>[2x]MSKIFDLVVIGAGSGGLEAAWNAATLYKKRVAVIDVQMVHGPPFFSALGGTCVNVGCVPKKLMVTGAQYMEHLRESAGFGWEFDRTTLRAEWKNLIAVKDEAVLNINKSYDEMFRDTEGLEFFLGWGSLESKNVVNVRESADPASAVKERLETEHILLASGSWPHMPNIPGIE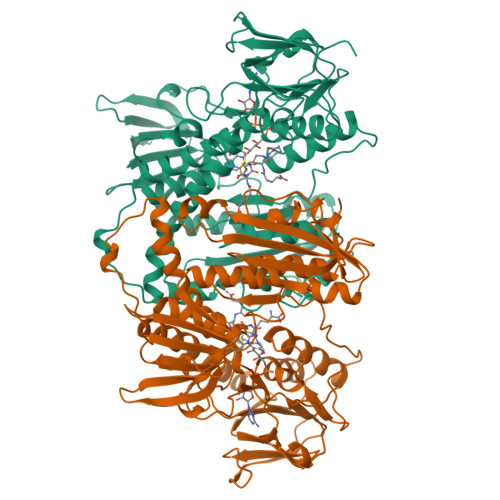HCISSNEAFYLPEPPRRVLTVGGGFISVEFAGIFNAYKPKDGQVTLCYRGEMILRGFDHTLREELTKQLTANGIQILTKENPAKVELNADGSKSVTFESGKKMDFDLVMMAIGRSPRTKDLQLQNAGVMIKNGGVQVDEYSRTNVSNIYAIGDVTNRVMLTPVAINEAAALVDTVFGTTPRKTDHTRVASAVFSIPPIGTCGLIEEVASKRYEVVAVYLSSFTPLMHKVSGSKYKTFVAKIITNHSDGTVLGVHLLGDNAPEIIQGIGICLKLNAKISDFYNTIGVHPTSAEELCSMRTPSYYYVKGEKMEKP N-[4-(1,1,1,3,3,3-hexafluoro-2-hydroxypropan-2-yl)phenyl]-N-[(4-phenoxyphenyl)methyl]benzenesulfonamide 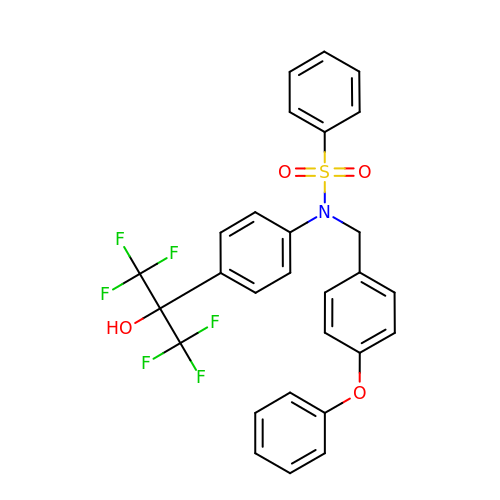| C28 H21 F6 N O4 S | OEAZXUIHXGZVAI-UHFFFAOYSA-N> MGSHHHHHHSSGLVPRGSHMFKREEIIEMANKDFEKAWIETKDLIKAKKINESYPRIKPVFGKTHPVNDTIENLRQAYLRMGFEEYINPVIVDERDIYKQFGPEAMAVLDRCFYLAGLPRPDVGLSDEKISQIEKLGIKVSEHKESLQKILHGYKKGTLDGDDLVLEISNALEISSEMGLKILEDVFPEFKDLTAVSSKLTLRSHMTSGWFLTVSDLMNKKPLPFKLFSIDRCFRREQKEDKSHLMTYHSASCAIAGEGVDINDGKAIAEGLLSQFGFTNFKFIPDEKKSKYYTPETQTEVYAYHPKLKEWLEVATFGVYSPVALSKYGIDVPVMNLGLGVERLAMISGNFADVREMVYPQFYEHKLNDRNVASMVKLDKVPVMDEIYDLTKELIESCVKNKDLKSPCELAIEKTFSFGKTKKNVKINIFEKEEGKNLLGPSILNEIYVYDGNVIGIPESFDGVKEEFKDFLEKGKSEGVATGIRYIDALCFKITSKLEEAFVSNTTEFKVKVPIVRSLSDINLKIDDIALKQIMSKNKVIDVRGPVFLNVEVKIEXXXXXX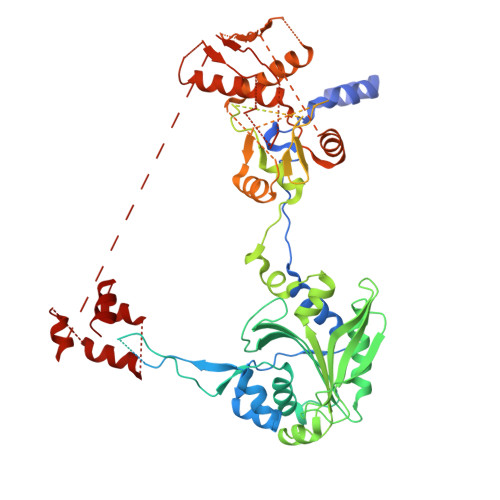XXXXXXXXXXXXXXXXXXXXXXXXXXXXXXXXXXXXXXXXXXXXXXXXXXXXXXXXXXXEXXXXXXXXXXXXXXXXXXXXXXXXXXXXXXXXXXXXXXXXXXXXXXXXXXXXXXXXXXXXXXX> MEQNPQSQLKLLVTRGKEQGYLTYAEVNDHLPEDIVDSDQIEDIIQMINDMGIQVMEEAPDADDLMLAENTADEDAAEAAAQVLSSVESEIGRTTDPVRMYMREMGTVELLTREGEIDIAKRIEDGINQVQCSVAEYPEAITYLLEQYDRVEAEEARLSDLITGFVDPNAEEDLAPTATHVGSELSQEDLDDDEDEDEEDGDDDSADDDNSIDPELAREKFAELRAQYVVTRDTIK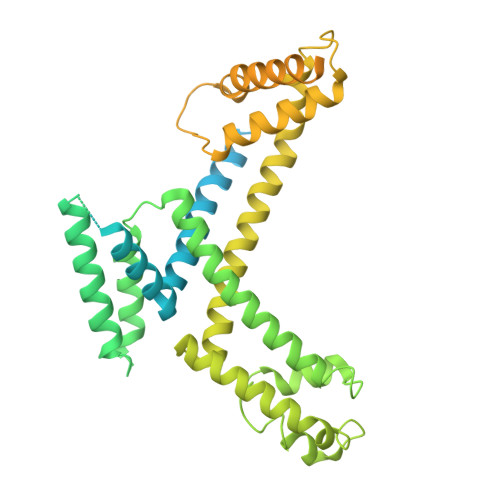AKGRSHATAQEEILKLSEVFKQFRLVPKQFDYLVNSMRVMMDRVRTQERLIMKLCVEQCKMPKKNFITLFTGNETSDTWFNAAIAMNKPWSEKLHDVSEEVHRALQKLQQIEEETGLTIEQVKDINRRMSIGEAKARRAKKEMVEANLRLVISIAKKYTNRGLQFLDLIQEGNIGLMKAVDKFEYRRGYKFSTYATWWIRQAITRSIADQARTIRIPVHMIETINKLNRISRQMLQEMGREPTPEELAERMLMPEDKIRKVLKIAKEPISMETPIGDDEDSHLGDFIEDTTLELPLDSATTESLRAATHDVLAGLTAREAKVLRMRFGIDMNTDYTLEEVGKQFDVTRERIRQIEAKALRKLRHPSRSEVLRSFLDD>AEIGGDHGYNATNIAAGQTSGAVTQIGPAVMGMVRRAIPNLIAFDICGVQPMNSPTGQVFALRAVYGKDPVAAGAKEAFHPMYGPDAMFSGQGAAKKFPALAASTQTTVGDIYTHFFQETGTVYLQASVQVTIDAGATDAAKLDA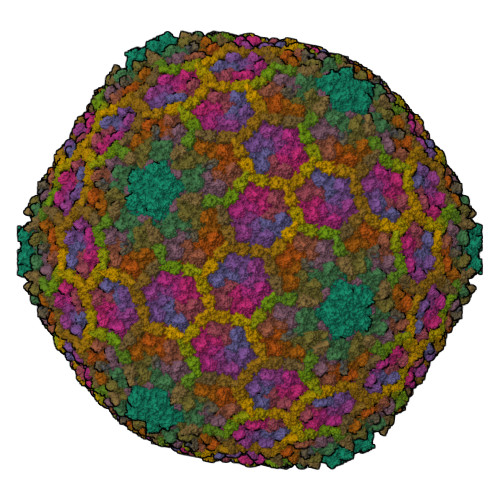EIKKQMEAGALVEIAEGMATSIAELQEGFNGSTDNPWNEMGFRIDKQVIEAKSRQLKAAYSIELTQDLRAVHGMDADAELSGILATEIMLEINREVVDWINYSAQVGKSGMTLTPGSKAGVFDFQDPIDIRGARWAGESFKALLFQIDKEAVEIARQTGRGEGNFIIASRNVVNVLASVDTGISYAAQGLATGFSTDTTKSVFAGVLGGKYRVYIDQYAKQDYFTVGYKGPNEMDAGIYYAPYVALTPLRGSDPKNFQPVMGFKTRYGIGINPFAESAAQAPASRIQSGMPSILNSLGKNAYFRRVYVKGI[12x];>[11x]MASARGYVNIKTFEQKLDGNKKIEGKEVSVAFPLYSDVHKISGAHYQTFPSEKAAYSTVYEENQRTEWIAANEDLWKVTG;> MTFTVDITPKTPTGVIDETKQFTATPSGQTGGGTITYAWSVDNVPQDGAEATFSYVLKGPAGQKTIKVVATNTLSEGGPETAEATTTITVKNKTQTTTLAVTPASPAAGVIGTPVQFTAALASQPDGASATYQWYVDDSQVGGETNSTFSYTPTTSGVKRIKCVAQVTATDYDALSVTSNEVSLTVNKKTMNPQVTLTPPSINVQQDASATFTANVTGAPEEAQITYSWKKDSSPVEGSTNVYTVDTSSVGSQTIEVTATVTAADYNPVTVTKTGNVTVTAKVAPEPEGELPYVHPLPHRSSAYIWCGWWVMDEIQKMTEEGKDWKTDDPDSKYYLHRYTLQKMMKDYPEVDVQESRNGYIIHKTALETGIIYTYP;> STTTNSNSIGRPNLVALTRATTKLIYSDIVATQRTNQPVAAFYGIKYLNPDNEFTFKTGATYAGEAGYVDREQITELTEESKLTLNKGDLFKYNNIVYKVLEDTPFATIEESDLELALQIAIVLLKVRLFSDAASTSKFESSDSEIADARFQINKWQTAVKSRKLKTGITVELAQDLEANGFDAPNFLEDLLATEMADEINKDILQSLITVSKRYKVTGITDSGFIDLSYASAPEAGRSLYRMVCEMVSHIQKESTYTATFCVASARAAAILAASGWLKHKPEDDKYLSQNAYGFLANGLPLYCDTNSPLDYVIVGVVENIGEKEIVGSIFYAPYTEGLDLDDPEHVGAFKVVVDPESLQPSIGLLVRYALSANPYTVAKDEKEARIIDGGDMDKMAGRSDLSVLLGVKLPKIIIDE An alternative, promising approach involves protein capsids, such as encapsulins, which can be viewed as genetically encoded enzyme encapsulation, and is particularly suitable for immobilization or within physiological conditions. The capsids, comprised of 60–240 subunits arranged in an icosahedral structure, engage with a conserved C-terminal encapsulin localization sequence (ELS), or a more extended N-terminal encapsulation-mediating domain, found on the guest protein. Our study showcases the encapsulation of the nitroreductase NfsB, which we produced as a fused dimer, within encapsulins.

Cryogenic electron microscopy reveals the overall architecture of the encapsulated dimeric NfsB within the nanoreactor environment and identifies multiple pore states in the shell. The crystal and cryo-EM structures of encapsulins from close homologs, have multiple openings in their capsid shells, including a threefold pore and an five-fold pore. These openings are thought to be the channels for the substrates and/or products of the cargo protein. The cryo-EM map in this area was ambiguous however and appears to be the superimposition of flexible states. To resolve this, the pentameric subunit was examined by 3-D classification and resulting volumes were refined using local refinement without symmetry constraints. This isolation a series of volumes that could be categorized as open, closed or uninterpretable. The open and closed particles were pooled and refined to yield complete, unambiguous maps (ESI†). The closed pore inner circle diameter in this structure was 4.62 Å. The primary drive of this is a shift in the pore forming loop (measuring 3.84 Å between the displaced His188 alpha carbon, see attached movies M1 and M2). The underlying cause of this movement is unclear and may represent an equilibrium of states when resting at cellular pH or could be a result of different packing states within the particles stacks.

>MNNLYRDLAPITESAWAEIELEATRTFKRHIAGRRVVDVSGPNGPTTASVSTGHLLDVSPPGDGVIAHLRDAKPLVRLRVPFTVARRDIDDVERGSQDSDWDPVKDAAKKLAFVEDRAIFEGYAAASIEGIRSSSSNPALALPDDAREIPDVIAQALSELRLAGVDGPYSVLLSAETYTKVSETTAHGYPIREHINRLVDGEIIWAPAIDGAFVLSTRGGDFDLQLGTDVSIGYLSHDAEVVHLYMEETMTFLCYTAEASVALTPELWSHPQFEK[60x]>PLGSVSEACPVCEKTVQNPCVLETGYVACYPCAISYLVNNE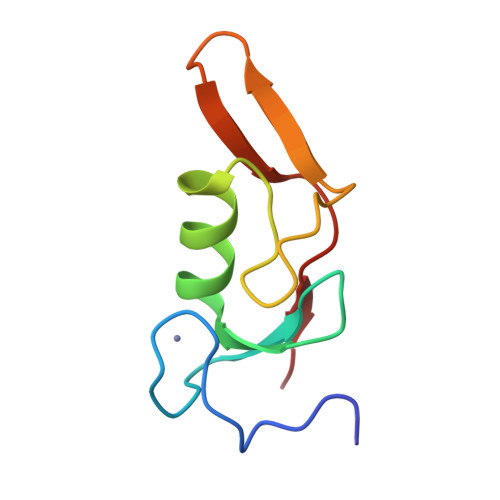GHCPVTNKKLLGCTYNKHTNKWEVVTGIRKLI[2x]(1,3-benzothiazol-2-yl)acetic acid | C9 H7 N O2 S 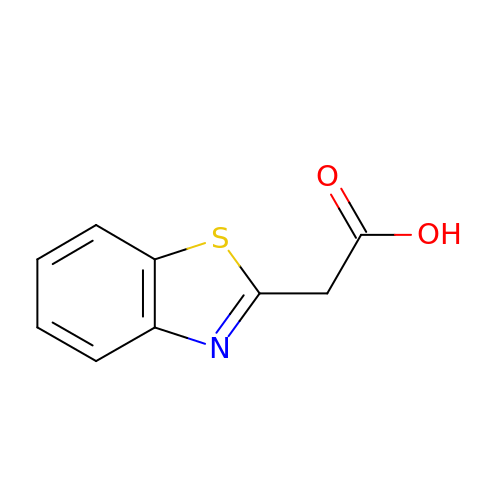| ZOAYQTSFMDZTQA-UHFFFAOYSA-N>[2x]AEAGITGTWYNQLGSTFIVTAGADGALTGTYESAVGNAESRYVLTGRYDSAP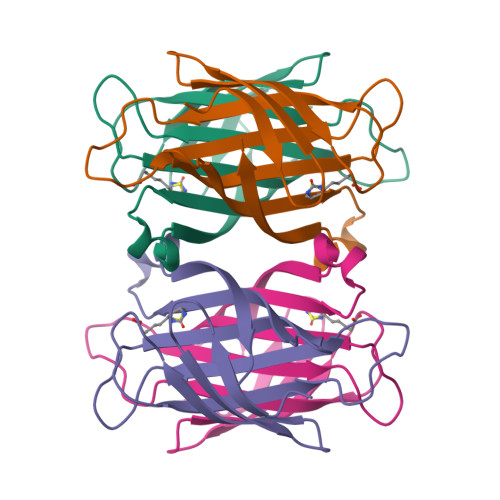ATDGSGTALGWTVAWKNNYRNAHSATTWSGQYVGGAEARINTQWLLTSGTTEANAWKSTLVGHATFTKVKPSAAS>INQVRPKLPLLKILHAAGAQGEMFTVKEVMHYLGQYIMVKQLYDQQEQHMVYCGGDLLGELLGR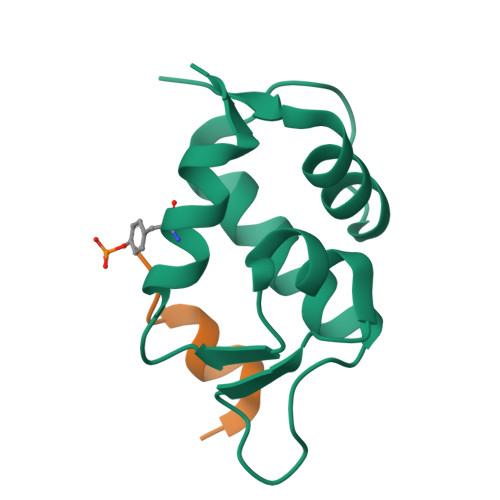QSFSVKDPSPLYDMLRKNLVT[2x];>TSFAEYWNLLSP[2x]>TYAFESNTNSVAASQMRNALNKLADSSKLDDAARAKFENELDSFFTLFRRYLVEKSSRTTLEWDKIKSPNPDEVVKYEIISQQPENVSNLSKLAVLKLNGGLGTSMGCVGPKSVIEVREGNTFLDLSVRQIEYLNRQYDSDVPLLLMNSFNTDKDTEHLIKKYSANRIRIRSFNQSRFPRVYKDSLLPVPTEYDSPLDAWYPPGHGDLFESLHVSGELDALIAQGREILFVSNGDNLGATVDLKILNHMIETGAEYIMELTDKTRADVKGGTLISYDGQVRLLEVAQVPKEHIDEFKNIRKFTNFNTNNLWINLKAVKRLIESSNLEMEIIPNQKTITRDGHEINVLQLETACGAAIRHFDGAHGVVVPRSRFLPVKTCSDLLLVKSDLFRLEHGSLKLDPSRFGPNPLIKLGSHFKKVSGFNARIPHIPKIVELDHLTITGNVFLGKDVTLRG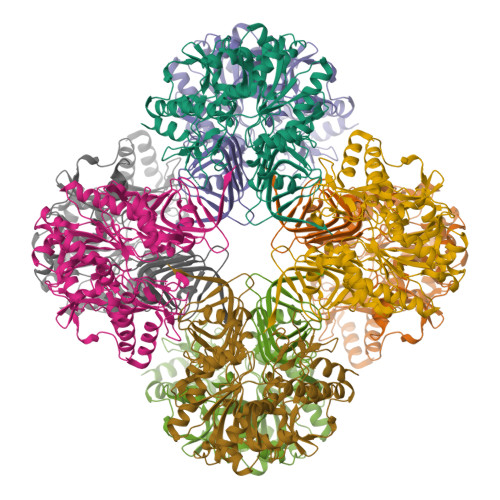TVIIVCSDGHKIDIPNGSILENVVVTGNLQILEH[2x]>MSVEGLGKDFCGAIIPDNFFPIEKLRNYTQMGLIRDFAKGSAVIMPGEEITSMIFLVEGKIKLDIIFEDGSEKLLYYAGGNSLIGKLYPTGNNIYATAMEPTRTCWFSEKSLRTVFRTDEDMIFEIFKNYLTKVAYYARQVAEMNTYNPTIRILRLFYELCSSQGKRVGDTYEITMPLSQKSIGEITG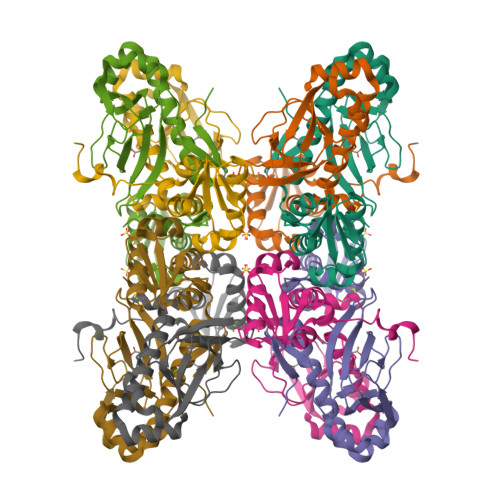VHHVTVSRVLACLKRENILDKKKNKIIVYNLGELKHLSEQTSYYSDPNSSSVDKLAAALDHH[2x]>MVMGNYQGKKAIVIGGTHGMGLATVRRLVEGGAEVLLTGRNESNIARIREEFGPRVHALRSDIADLNEIAVLGAAAGQTLGAIDLLHINAGVSELEPFDQVSEASYDRQFAVNTKGAFFTVQRLTPLIREGGSIVFTSSVADEG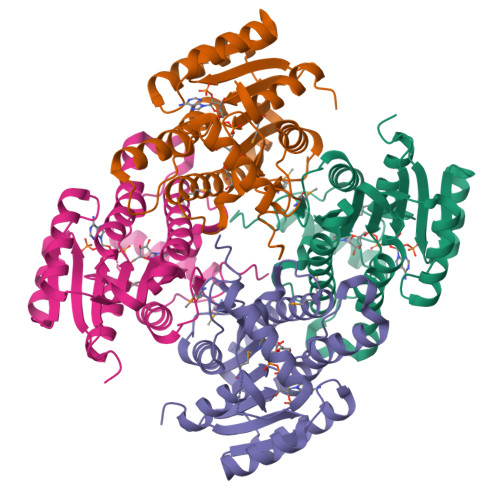GHPGMSVYSASKAALVSFASVLAAELLPRGIRVNSVSPGFIDTPTKGVAGITEAERAEFKTLGDNITPMKRNGTADEVARAVLFLAFEATFTTGAKLAVDGGLGQKLSTAA[4x]>MDHLPIFCQLRDRDCLIVGGGDVAERKARLLLEAGARLTVNALTFIPQFTVWANEGMLTLVEGPFDETLLDSCWLAIAATDDDTVNQRVSDAAESRRIFCNVVDAPKAASFIMPSIIDRSPLMVAVSSGGTSPVLARLLREKLESLLPQHLGQVARYAGQLRARVKKQFATMGERRRFWEKFFVNDRLAQSLANADEKAVNATTERLFSEPLDHRGEVVLVGAGPGDAGLLTLKGLQQIQQADIVVYDRLVSDDIMNLVRRDADRVFVGKRAGYHCVPQEEINQILLREAQKGKRVVRLKGGDPFIFGRGGEELETLCHAGIPFSVVPGITAASGCSAYSGIPLTHRDYAQSVRLVTGHLKTGGELDWENLAAEKQTLVFYMGLNQAATIQEKLIAFGMQADMPVALVENGTSVKQRVVHGVLTQLGELAQQVE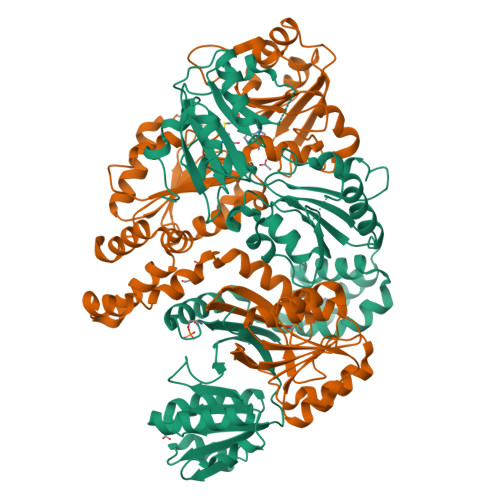SPALIIVGRVVALRDKLNWFSNH[2x]>[2x]DWVIPPISCPENEKGEFPKNLVQIKSNRDKETKVFYSITGQGADKPPVGVFIIERETGWLKVTQPLDREAIAKYILYSHADSSNGEAVEDPMEI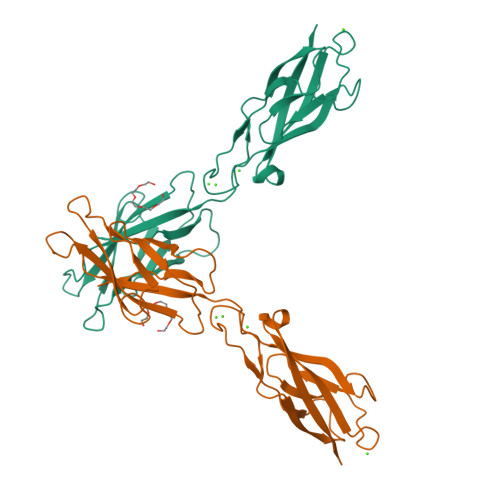VITVTDQNDNRPEFTQEVFEGSVAEGAVPGTSVMKVSATDADDDVNTYNAAIAYTIVSQDPELPHKNMFTVNRDTGVISVLTSGLDRESYPTYTLVVQAADLQGEGLSTTAKAVITVKD> MGHHHHHHGSLVPRGSEYDYLFKLLLIGNSGVGKSCLLLRFSDDTYTNDYISTIGVDFKIKTVELDGKTVKLQIWDTAGQERFRTITSSYYRGSH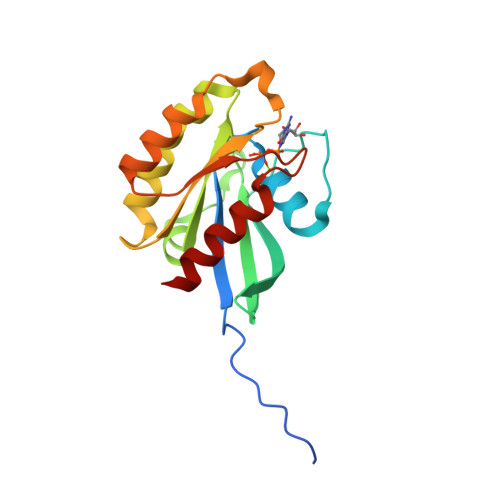GIIIVYDVTDQESFNGVKMWLQEIDRYATSTVLKLLVGNKCDLKDKRVVEYDVAKEFADANKMPFLETSALDSTNVEDAFLTMARQIKES> GAMTFTRYSRLRVIAEIRHGDIFHSANIVSSIEFDRDDELFATAGVSRCIKVFDFSSVVNEPADMQCPIVEMSTRSKLSCLSWNKHEKNHIASSDYEGIVTVWDVTTRQSLMEYEEHEKRAWSVDFSRTEPSMLVSGSDDCKVKVWCTRQEASVINIDMKANICCVKYNPGSSNYIAVGSADHHIHYYDLRNISQPLHVFSGHKKAVSYVKFLSNNELASASTDSTLRLWDVKDNLPVRTFRGHTNEKNFVGLTVNSEYLACGSETNEVYVYHKEITRPVTSHRFGSPDMDDAEEEAGSYFISAVCWKSDSPTMLTANSQGTIKVLVLAA;> XELLMVPDMY

The COP1 E3 ubiquitin ligase is a central signaling hub that integrates inputs from plant light‐sensing photoreceptors. COP1 contains an N‐terminal zinc finger, a central coiled‐coil, and a C‐terminal WD40 domain, which is essential for proper COP1 function (Deng et al, 1992; McNellis et al, 1994). COP1 regulates gene expression and plays a central role as a repressor of photomorphogenesis by directly modulating the stability of transcription factors that control the expression of light‐regulated genes.

We mapped putative VP motifs in all these proteins and assessed their binding affinities to the COP1 WD40 domain. We could detect binding for most of the peptide motifs in ITC assays, with dissociation constants in the mid‐micromolar range (Figs 4A and EV4). Next, we obtained crystal structures for the different peptides bound to COP1 (1.3–2.0 Å resolution, see Tables EV1 and EV2, and EV4) to compare their peptide binding modes. We found that all peptides bind in a similar configuration with the VP forming the center of the binding site (r.m.s.d. between the different peptides range from ~ 0.3 to 1.5 Å, comparing 5 or 6 corresponding Cα atoms). In yeast 3‐hybrid assays, we find that, similar to HY5, UV‐B‐activated UVR8 can efficiently compete with HYH and an N‐terminal fragment of HFR1 for binding to COP1 (Fig EV5).> MLTPTPDSSPRSTSSPSQSKNGSFTPRTANI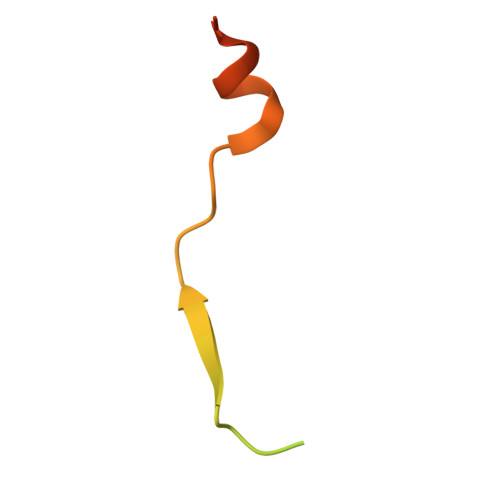LKPLMSPPSREEIMATLLDHD>[12x]MKAAESLPNIQIKSIAGITEPTILQYFATLNAGEFAATAALFAVDGVMYPPFESGIVGPDAIA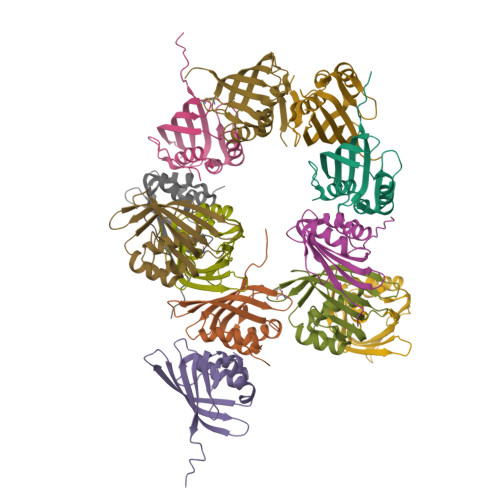AYLQQEAQGIKAEPQQGLAETSEDGHTQVQVSGKAQTSWCGVNVLWLFTLNQEKQIIHTQIKLLASPQELLALRREQ>[2x]NVAELKKSFNRHLHFTLVKDRNVATTRDYYFALAHTVRDHLVGRWIRTQQHYYDKCPKRVYYLSLEFYMGRTLQNTMINLGLQNACDEAIYQLGLDIEELEEIEEDAGLGNGGLGRLAACFLDSMATLGLAAYGYGIRYEYGIFNQKIRDGWQVEEADDWLRYGNPWEKSRPEFMLPVHFYGKVE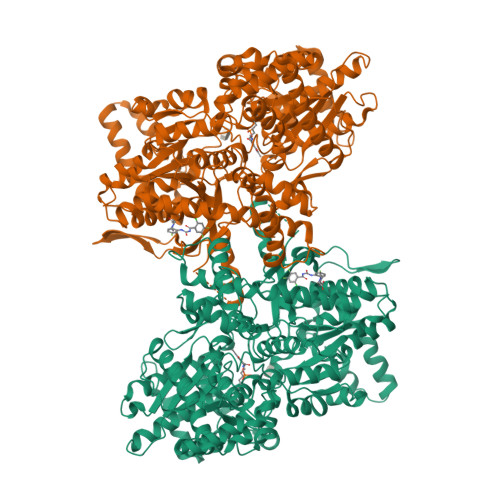HTNTGTKWIDTQVVLALPYDTPVPGYMNNTVNTMRLWSARAPNDFNLRDFNVGDYIQAVLDRNLAENISRVLYPNDNFFEGKELRLKQEYFVVAATLQDIIRRFKASKFGSTRGAGTVFDAFPDQVAIQLNDTHPALAIPELMRIFVDIEKLPWSKAWELTQKTFAYTNHTVLPEALERWPVDLVEKLLPRHLEIIYEINQKHLDRIVALFPKDVDRLRRMSLIEEEGSKRINMAHLCIVGSHAVNGVAKIHSDIVKTKVFKDFSELEPDKFQNKTNGITPRRWLLLCNPGLAELIAEKIGEDYVKDLSQLTKLHSFLGDDVFLRELAKVKQENKLKFSQFLETEYKVKINPSSMFDVQVKRIHEYKRQLLNCLHVITMYNRIKKDPKKLFVPRTVIIGGKAAPGYHMAKMIIKLITSVADVVNNDPMVGSKLKVIFLENYRVSLAEKVIPATDLSEQISTAGTEASGTGNMKFMLNGALTIGTMDGANVEMAEEAGEENLFIFGMRIDDVAALDKKGYEAKEYYEALPELKLVIDQIDNGFFSPKQPDLFKDIINMLFYHDRFKVFADYEAYVKCQDKVSQLYMNPKAWNTMVLKNIAASGKFSSDRTIKEYAQNIWNVEPSD> SVTSAKVAVNGVQLHYQQTGEGDHAVLLLPGMLGSGETDFGPQLKNLNKKLFTVVAWDPRGYGHSRPPDRDFPADFFERDAKDAVDLMKALKFKKVSLLGWSDGGITALIAAAKYPSYIHKMVIWGANAYVTDEDSMIYEGIRDVSKWSERTRKPLEALYGYDYFARTCEKWVDGIRQFKHLPDGNICRHLLPRVQCP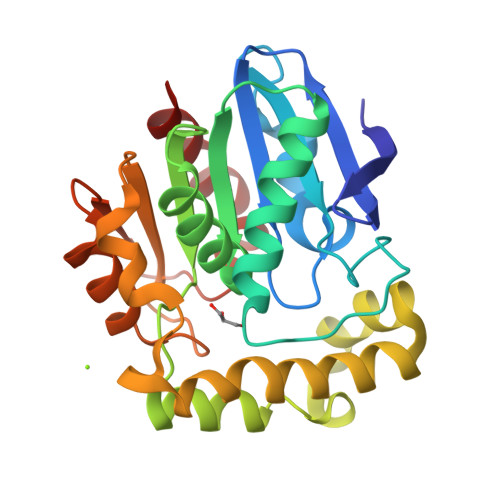ALIVHGEKDPLVPRFHADFIHKHVKGSRLHLMPEGKHNLHLRFADEFNKLAEDFLQ Fpg/Nei DNA glycosylases are composed of two globular domains, an N-terminal domain rich in beta-structures and a C-terminal domain rich in alpha-structures. Most of them contain an original zinc finger (ZnF) motif (defining a new class of ZnF) comprising a β-hairpin structure with generally four cysteine residues coordinating the Zn2+ ion (type –C-X2(3)-C(H)-X16-18-C-X2-C-). Only the bacterial Fpg enzymes can excise 8-oxoG, the major oxidation product of purines. To further our understanding of the TXn mode of action, we solved several crystal structures of LlFpg bound to 14-mer [THF:C] (LRC) in the presence of thio-compounds.

Using this method, we successfully resolved the structures of LRC with the moderately potent inhibitor 2TX (new crystal structure), high-efficiency inhibitors TX13, TX19, TX20, TX27, low-efficiency inhibitor TX15 and, TX19 in the presence of TCEP. A similar non-covalent binding at site II is also observed with TXn. The strictly conserved residues R260 of the ZnF loop and K57 of the β2-β3 loop of the N-terminal LlFpg domain are directly involved in the recognition of 2TX/TXn. The guanidinium group of the R260 side chain interacts with the unique sulfur atom of 2TX, TX15, TX20 and TX27, with the sulfur atom at the C8 position of TX19 (with or without TCEP) or with the N1 atom of the purine moiety of TX13. The epsilon amino group of the K57 side chain interacts with the sulfur atom of all 2TX/TXn compounds. Through binding at site II, the present crystal structures indicate that 2TX/TXn in their reduced forms do not disturb the local structure of the complex (the DNA backbone conformation and the side chain orientation of R260 and K57 are unchanged). Indeed, fine inspection of the crystal structures of C2 with that of the lesion recognition complex C1 resolved in the presence of 2TX, TX13, TX15, TX19, TX20 and TX27 showed that the 5′-overhanging cytosine of the damage-containing strand recognized by the second molecule (Mol-2) of LlFpg in C2 clashes with 2TX/TXn bound at the site II.

> PELPEVETVRRELEKRIVGQKIISIEATYPRMVLTGFEQLKKELTGKTIQGISRRGKYLIFEIGDDFRLISHLRMEGKYRLATLDAPREKHDHLTMKFADGQLIYADVRKFGTWELISTDQVLPYFLKKKIGPEPTYEDFDEKLFREKLRKSTKKIKPYLLEQTLVAGLGNIYVDEVLWLAKIHPEKETNQLIESSIHLLHDSIIEILQKAIKLGGSSIRTYSALGSTGKMQNELQVYGKTGEKCSRCGAEIQKIKVAGRGTHFCPVCQQK>[2x]MPPETATNPKDARHDGWQTLKRFLPYLWPADNAVLRRRVVGAILMVLLGKATTLALPFAYKKAVDAMTLGGG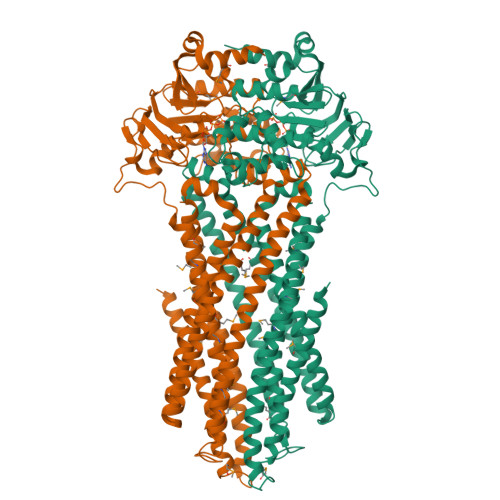AQPALTVALAFVLAYALGRFSGVLFDNLRNIVFERVGQDATRHLAENVFARLHKLSLRFHLARRTGEVTKVIERGTKSIDTMLYFLLFNIAPTVIELTAVIVIFWLNFGLGLVTATILAVIAYVWTTRTITEWRTHLREKMNRLDGQALARAVDSLLNYETVKYFGAESREEARYASAARAYADAAVKSENSLGLLNIAQALIVNLLMAGAMAWTVYGWSQGKLTVGDLVFVNTYLTQLFRPLDMLGMVYRTIRQGLIDMAEMFRLIDTHIEVADVPNAPALVVNRPSVTFDNVVFGYDRDREILHGLSFEVAAGSRVAIVGPSGAGKSTIARLLFRFYDPWEGRILIDGQDIAHVTQTSLRAALGIVPQDSVLFNDTIGYNIAYGRDGASRAEVDAAAKGAAIADFIARLPQGYDTEVGERGLKLSGGEKQRVAIARTLVKNPPILLFDQATSALDTRTEQDILSTMRAVASHRTTISIAHRLSTIADSDTILVLDQGRLAEQGSHLDLLRRDGLYAEMWARQAAESAEVSEAAEHHHHHH>ALRDRVKKLKLLIMDIDGVLTDGKLYYTEHGETIKVFNVLDGIGIKLLQKMGITLAVISGRDSAPLITRLKELGVEEIYTGSYKKLEIYEKIKEKYSLKDEEIGFIGDDVVDIEVMKKVGFPVAVRNAVEEVRKVAVYITQRNGGEGALREVAE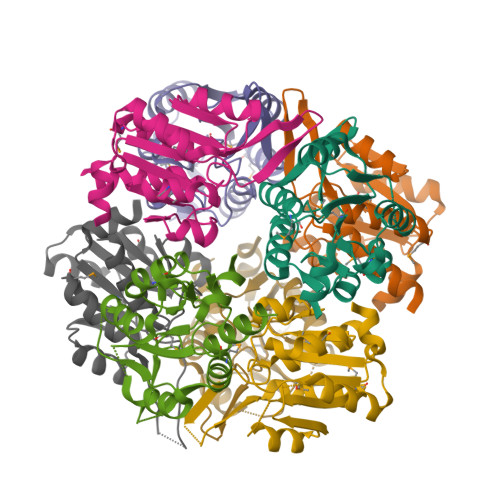LIHFLKND[8x]> MGGKSNGEKKYIVGFKQGFKSCAKKEDVISEKGGKLQKCFKYVDAASATLNEKAVEELK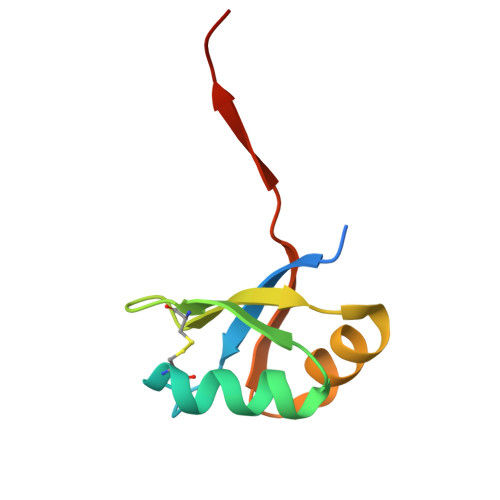KDPSVAYVEEDKLYRALSATS> MASSRCPAPRGCRCLPGASLAWLGTVLLLLADWVLLRTALPRIFSLLVPTALPLLRVWAVGLSRWAVLWLGACGVLRATVGSKSENAGAQGWLAALKPLAAALGLALPGLALFRELISWGAPGSADSTRLLHWGSHPTAFVVSYAAALPAAALWHKLGSLWVPGGQGGSGNPVRRLLGCLGSETRRLSLFLVLVVLSSLGEMAIPFFTGRLTDWILQDGSADTFTRNLTLMSILTIASAVLEFVGDGIYNNTMGHVHSHLQGEVFGAVLRQETEFFQQNQTGNIMSRVTEDTSTLSDSLSENLSLFLWYLVRGLCLLGIMLWGSVSLTMVTLITLPLLFLLPKKVGKWYQLLEVQVRESLAKSSQVAIEALSAMPTVRSFANEEGEAQKFREKLQEIKTLNQKEAVAYAVNSWTTSISGMLLKVGILYIGGQLVTSGAVSSGNLVTFVLYQMQFTQAVEVLLSIYPRVQKAVGSSEKIFEYLDRTPRCPPSGLLTPLHLEGLVQFQDVSFAYPNRPDVLVLQGLTFTLRPGEVTA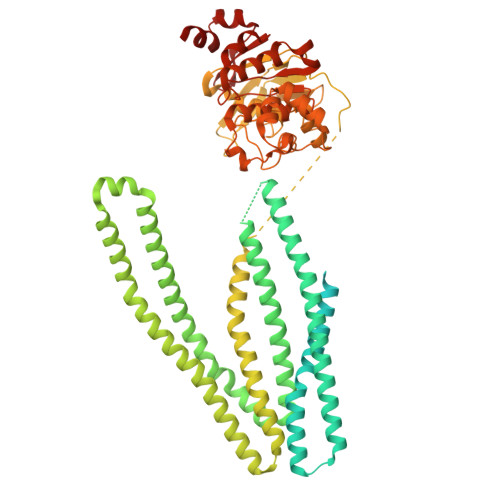LVGPNGSGKSTVAALLQNLYQPTGGQLLLDGKPLPQYEHRYLHRQVAAVGQEPQVFGRSLQENIAYGLTQKPTMEEITAAAVKSGAHSFISGLPQGYDTEVDEAGSQLSGGQRQAVALARALIRKPCVLILDDATSALDANSQLQVEQLLYESPERYSRSVLLITQHLSLVEQADHILFLEGGAIREGGTHQQLMEKKGCYWAMVQAPADAPE> ATMALKTVDAKQTTSVCCYCSVGCGLIVHTDKKTNRAINVEGDPDHPINEGSLCAKGASTWQLAENERRPANPLYRAPGSDQWEEKSWDWMLDTIAERVAKTREATFVTKNAKGQVVNRCDGIASVGSAAMDNEECWIYQAWLRSLGLFYIEHQARIUHSATVAALAESYGRGAMTNHWIDLKNSDVILMMGSNPAENHPISFKWVMRAKDKGATLIHVDPRYTRTSTKCDLYAPLRSGSDIAFLNGMTKYILEKELYFKDYVVNYTNASFIVGEGFAFEEGLFAGYNKETRKYDKSKWGFERDENGNPKRDETLKHPRCVFQIMKKHYERYDLDKISAICGTPKELILKVYDAYCATGKPDKAGTIMYAMGWTQHTVGVQNIRAMSINQLLLGNIGVAGGGVNALRGEANVQGSTDHGLLMHIYPGYLGTARASIPTYEEYTKKFTPVSKDPQSANWWSNFPKYSASYIKSMWPDADLNEAYGYLPKGEDGKDYSWLTLFDDMFQGKIKGFFAWGQNPACSGANSNKTREALTKLDWMVNVNIFDNETGSFWRGPDMDPKKIKTEVFFLPCAVAIEKEGSISNSGRWMQWRYVGPEPRKNAIPDGDLIVELAKRVQKLLAKTPGKLAAPVTKLKTDYWVNDHGHFDPHKIAKLINGFALKDFKVGDVEYKAGQQIATFGHLQADGSTTSGCWIYTGSYTEKGNMAARRDKTQTDMQAKIGLYPGWTWAWPVNRRIIYNRASVDLNGKPYAPEKAVVEWNAAEKKWVGDVPDGPWPPQADKEKGKRAFIMKPEGYAYLYGPGREDGPLPEYYEPMECPVIEHPFSKTLHNPTALHFATE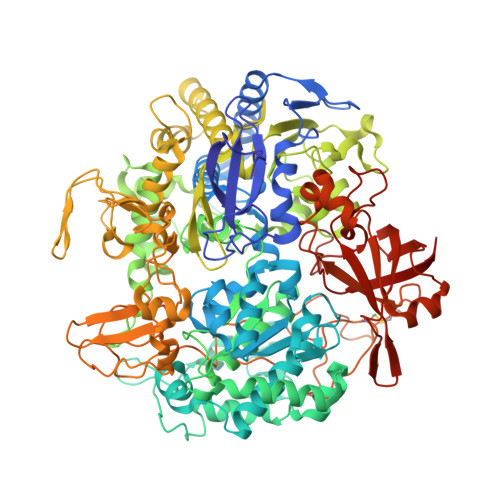EKAVCDPRYPFICSTYRVTEHWQTGLMTRNTPWLLEAEPQMFCEMSEELATLRGIKNGDKVILESVRGKLWAKAIITKRIKPFAIQGQQVHMVGIPWHYGWSFPKNGGDAANILTPSVGNPNTGIPETKAFMVNVTKA>[2x]GPHMEEIMQSDSKIEKMLPDGGRLVVFPNGTRKELSADGQTVKVMFFNGDVKHTMPDQRVIYYYAEAQTTHITYPDGMEVLQFPNNQTEKHFPDGRKEITFPDQTVKTLHPDGREESVLTDGTIIQLNPDGSKVIQFNTGQREIHTADFKRREYPDGTVKTVYSDGRQETQYPTGRVRLKDPQGKVIMDTKA;>GSGVEDEDLSPRPSPNPHPVSQENLYFQ[2x]

Of particular interest in this regard is the putative centriolar CPAP–STIL complex, as mutations in both components result in MCPH. CPAP and STIL are strictly required for centriole assembly: STIL at a very early stage and CPAP slightly later, possibly by controlling the organisation and length of the centriolar microtubules. Instead, we demonstrate that the TCP domain of CPAP constitutes a novel proline-rich-motif (PRM) recognition-domain that specifically binds to a short target motif in STIL. Our mutational analysis of the interface demonstrates a remarkable correlation between the ability of mutant proteins to bind to one another in vitro and their ability to support centriole assembly in vivo, providing compelling support for our structural model of the metazoan CPAP–STIL complex. These data strongly suggest that the interaction between CPAP and STIL is a conserved, essential step in centriole biogenesis.

To understand how CPAP and STIL interact at the molecular level, we obtained the crystal structures of the TCP-domain of D. rerio CPAP937–1124, both on its own and in a complex with D. rerio STIL408–428. In both structures, the TCP domain adopts a nearly identical conformation, suggesting that no significant conformational change occurs in CPAP upon binding to STIL (RMSD = 1.5 Å ± 0.2 Å over 148 ± 4 Cα pairs). The structure of the CPAP–STIL complex revealed that the STIL peptide binds in a polyproline II helical conformation along one edge of the TCP domain β-sheet. The STIL peptide binds to CPAP by four main mechanisms. First, three STIL prolines (P417, P421, and P423) pack against aromatic CPAP residues (F978, Y996, and F1015) in a way that resembles target motif recognition by other described proline-rich motif (PRM) binding domains. Second, R418 (STIL) makes a cation-π interaction with the phenyl ring of Y994 (CPAP). Third, STIL R418 is further involved in a water-mediated hydrogen bonding network that includes CPAP residues H1003 and T1005. Finally, sidechain–mainchain interactions are formed between CPAP residues Y994, Q1019, and E1021 and the bound STIL peptide. The CPAP and STIL residues involved in this interaction are highly conserved across metazoans. We conclude that the TCP domain of CPAP adopts a unique extended open β-sheet conformation that recognises a series of conserved prolines in the CR2 region of STIL.3-benzoylbenzoic acid | C14 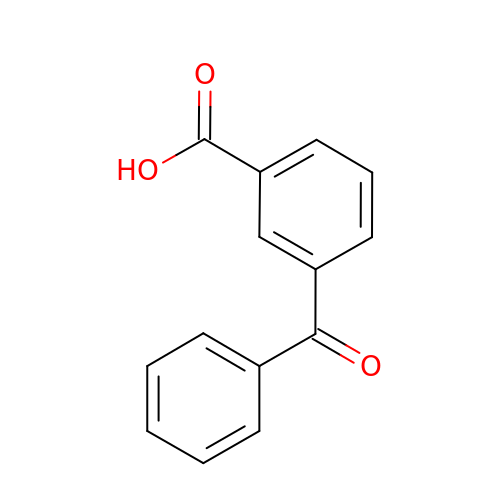H10 O3 | AXJXRLHTQQONQR-UHFFFAOYSA-N> MDNKSAVSALQEFCARTQINLPTYSFIPGEDGGYVCKVELLEIEALGNGRSKRDAKH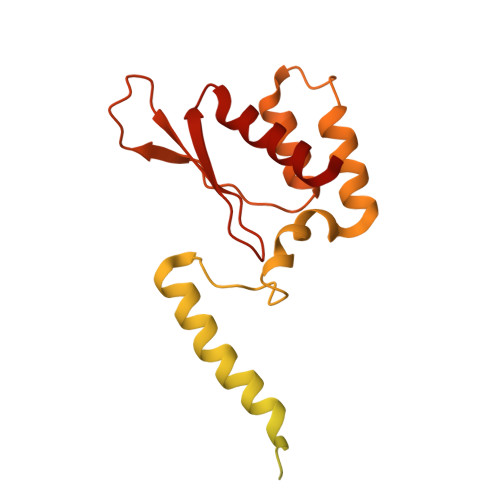LAASNILRKIQLLPGIHGLMKDSTVGDLDEELTNLNRDMVKELRDYCVRREMPLPCIEVVQQSGTPSAPEFVACCSVASIVRYGKSDKKKDARQRAAIEMLALISSNSDNLRPDQMQVASTSKLKVVDMEESMEELEALRRKKFTTYWELKEAGSVDHTGMRLCDRHNYFKNFYPTLKKEAIEAINSDEYESSKDKAMDVMSSLKITPKISEVESSSLVPLLSVELNCAFDVVLMAKETDIYDHIIDYFRTMLI> DGAKIYAQCAGCHQQNGQGIPGAFPPLAGHVAEILAKEGGREYLILVLLYGLQGQIEVK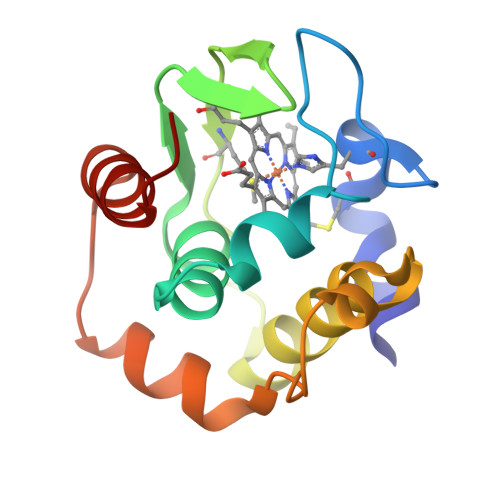GMKYNGVMSSFAQLKDEEIAAVLNHIATAWGDAKKVKGFKPFTAEEVKKLRAKKLTPQQVLAERKKLGLK>PVTKTRLIDTPVRSGQRIYAPQCDLIVTSHVSAGAELIADGNIHVYGMMRGRALAGASGDRETQIFCTNLMAELVSIAGEYWLSDQIPAEFYGKAARLQLVENALTVQPLNLEHHHHHH[2x]

In the Gram-negative bacterium E. coli, a tubulin like protein (FtsZ) polymerizes at mid-cell to form a ring structure (Z-ring) to ensure cell division, which is often spatially regulated by the Min system, including MinC, MinD and MinE, through a pole-to-pole oscillation. MinC, as an inhibitor of the Z-ring, is recruited to the membrane by MinD and prevents FtsZ polymerization. The C-terminal domain of MinC interacts with MinD, while its N-terminal domain directly inhibits FtsZ filamentation. In E. coli, MinC and MinD undergo a rapid pole-to-pole oscillation in response to MinE, which causes a periodic block of the polar division sites.

In this work, we determined the crystal structure of the dimeric C-terminal domain of MinC from E. coli (EcMinCCTD). The crystal structure of EcMinCCTD was solved at 3.0 Å resolution using the molecular replacement method. EcMinCCTD forms a dimer within the asymmetric unit via domain swapping. EcMinCCTD forms a dimer between the two β-sheets in each subunit, as observed in the TmMinCCTD structure. The tight dimer formed through the MinCCTD beta helical domain is similar to that of TmMinCCTD (left). The two MinCCTD structures superimposed with a root-mean-square deviation (RMSD) of 1.4 Å for the 110 Cα atoms (residues 122–231). Compared to AaMinCCTD, EcMinCCTD and TmMinCCTD both lack a helix3 at its C-terminus. SDS-PAGE analysis of the harvested crystals showed that these crystals resulted from a degradation fragment of the MinC protein at a molecular weight of ~13 kD. Furthermore, western blotting results demonstrated that this fragment of MinC had the C-terminal 6 × His tag (data not shown), which suggested that our crystals were from EcMinC’s C-terminal domain (MinCCTD). This is likely caused by degradation of the flexible linker between the N- and C-terminal domains of MinC, which is easily susceptible to non-specific proteolysis. As a result, we went back to the initial method of using full-length MinC to obtain MinCCTD crystals. It is inferred that MinCNTD, although cleaved off over time, initially helps to promote the correct folding and solubility of MinCCTD. In this EcMinCD model structure, the RSGQ motif of MinC and MinD’s helix 7 make up an interaction interface as expected.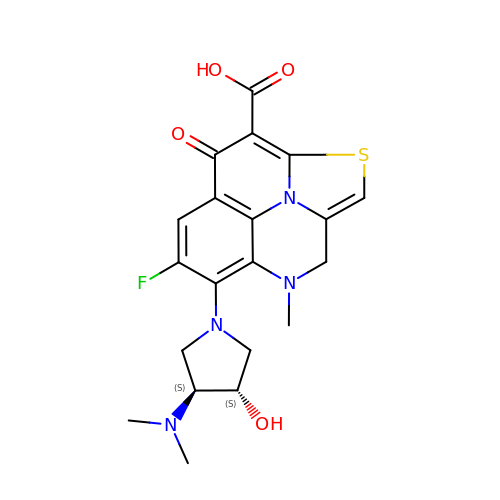5-[(3S,4S)-3-(dimethylamino)-4-hydroxypyrrolidin-1-yl]-6-fluoro-4-methyl-8-oxo-3,4-dihydro-8H-1-thia-4,9b-diazacyclopenta[cd]phenalene-9-carboxylic acid | C20 H21 F N4 O4 S | JHSMWPKZVMQLKB-STQMWFEESA-N> GPHMGGSMQKVSLRVTPRLVLEVNRHNAICVATNVPEFYNARGDLNIRDLRAHVKARMISSQFCGYVLVSLLDSEDQVDHLNIFPHVFSERMILYKPNNVNLMEMCALLSMIENAKSPSIGLCREVLGRL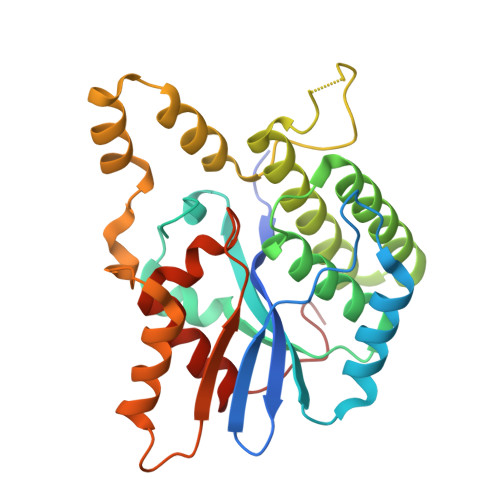TLLHSKCNNLDSLFLYNGARTLLSTLVKYHDLEEGAATPGPWNEGLSLFKLHKELKRAPSEARDLMQSLFLTSGKMGCLARSPKDYCADLNKEEDANSGFTFNLFYQDSLLTKHFQCQTVLQTLRRKCLGSDTVSKIIP> GSEVSEEELKNFSGPVPDLPEGITVAYTIPKKQEDSV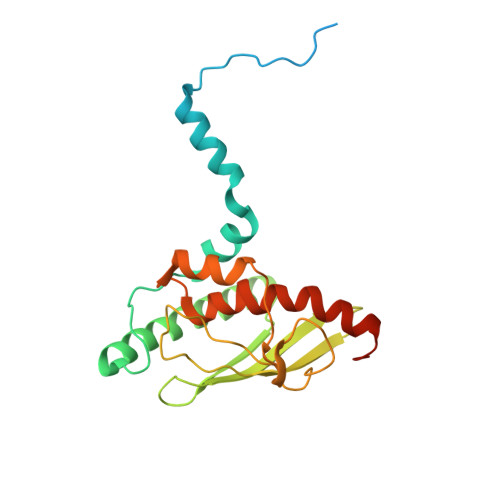TELTVEDSGESLEDLMAKMKNMMADEATRRVVSEIPVLKTNAGPRDRELWVQRLKEEYQSLIRYVENNKNADNDWFRLESNKEGTRWFGKCWYIHDLLKYEFDIEFDIPITYPTTAPEIAVPELDGKTAKMYRGGKICLTDHFKPLWARNVPKFGLAHLMALGLGPWLAVEIPDLIQKGVIQHKEKCNQ>ANVRLQHHHHHHHLEANPNQQTEDEWKFTLKNAYINRDFDNDALKDTGSWSQAASLFYKSKMHDTPLVIADKPITIGADASVQYAVRLSSDKHVADTVLPFNKETQSQASDYLKYGATLKLGYDKTLLSVGELWLDLPVTAVDASRQLLTSYWGTNLKS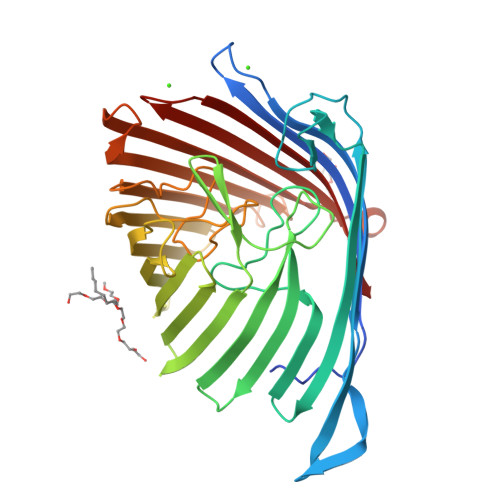QLSDQLYAEIGRVEKVSPRNEEDFKKFSFTANGITKESDGLNYIDLRYQFTPSLKGEYYFGNLEDLYNKHYVGLEHTWKQPTFALTSKFKYFNAKDDGNTFDIDAENIGLLETVKVKNHTFGLGYQQIIGESAYPLPDGFLPETYFINWNATGFFKEDEKSYHVMYGYDFKDYIPGLNAMVKYVYGHDFKAANGEKNHETESNVILNYAFQQPLLKGFALQYIRIDYNVKHGNDFGEDRLFVNYTKKF[2x]>[2x]GAMARKELSSLEELFRHYGVRYMTLTKMVEMGFTVNTLVNMTEQELDDVIRTLVDI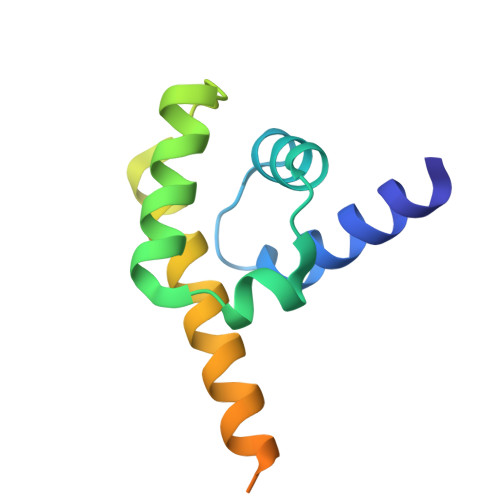YRVDLLVGEKYGIKSAVRAEKRRLDELERKKLDLFVDVDGKRKADENALDTLSQ Trypanothione reductase (TR) is a suitable target for drug discovery approaches against leishmaniasis, although the identification of potent inhibitors is still challenging. TR structure from different protozoan parasites has been extensively characterized by crystallography, showing that all key residues are conserved. This homodimeric flavoenzyme possesses four cavities binding two nicotinamide adenine dinucleotide phosphate hydrogen (NADPH) and two trypanothione molecules. Each NADPH cavity is separated from the trypanothione active site by a flavin adenine dinucleotide (FAD) cofactor allowing the transfer of two electrons by the participation of two catalytic cysteines (C52 and C57) which, together with H461′, E466′, and E467′ of the γ-Glu site, form the catalytic machinery. The active site features a hydrophobic cleft, named mepacrine binding site (MBS) after the crystal structure with the mepacrine inhibitor was solved.

To validate the predicted binding mode for further rational structure-based drug design and ligand optimization, the structures of TbTR with the most promising compounds 9, 10, and 14 were determined by X-ray crystallography. The effect of N-piperazine substitution on binding affinity was assessed by introducing a methyl or a diClBn group in B to afford quaternary ammonium salts 9 and 10, respectively. Quaternization of the piperazine promotes improvement in IC50 values compared to that of 5 (IC50 = 54.6 μM) by about 3-fold for 9 (IC50 = 20.5 μM), 42-fold for 10 (IC50 = 1.31 μM), and 23-fold for 14 (IC50 = 2.35 μM). However, this improvement does not seem to relate to the interaction between the positively charged ammonium and the protein but as shown in the solved structures, rather to the larger inhibitor structures, more efficiently occupying the binding pocket. Remarkably, 10, endowed with a completely new chemotype and a Ki value of 0.2 μM, stands among the most effective LiTR inhibitors so far developed. The densities observed inside the trypanothione pocket for both TR dimers provided well-defined results for some portions of the compounds, namely, the ethyl-p-fluorophenyl and furan moieties, indicating that these common portions anchor 9, 10, and 14 to the Z-site by van der Waals and electrostatic interactions, as previously observed for fragment. From the interaction network, it is clear that the furan and the ethyl-p-fluorophenyl groups anchor 9, 10, and 14 to the Z-site, consistently with the binding of the initial fragments. It is also evident that the dichlorobenzyl group—when present—protrudes toward the MBS together with the phenylpropyl moiety, making a T-shaped π-stacking interaction with W21. With regard to selectivity, the binding of the optimized fragments 10 and 14 is probably allowed for hGR despite the presence of the bulkier side chains in hGR compared to those in TR.

>[4x]GSHMSKAFDLVVIGAGSGGLEAGWNAATLYGKRVAVVDVQTSHGPPFYAALGGTCVNVGCVPKKLMVTGAQYMDHLRESAGFGWEFDGSSVKANWKKLIAAKNEAVLDINKSYEGMFNDTEGLDFFLGWGSLESKNVVVVRETADPKSAVKERLQADHILLATGSWPQMPAIPGIEHCISSNEAFYLPEPPRRVLTVGGGFISVEFAGIFNAYKPPGGKVTLCYRNNLILRGFDETIREEVTKQLTANGIEIMTNENPAKVSLNTDGSKHVTFESGKTLDVDVVMMAIGRIPRTNDLQLGNVGVKLTPKGGVQVDEFSRTNVPNIYAIGDITDRLMLTPVAINEGAALVDTVFGNKPRKTDHTRVASAVFSIPPIGTCGLIEEVAAKEFEKVAVYMSSFTPLMHNISGSKYKKFVAKIVTNHSDGTVLGVHLLGDGAPEIIQAVGVCLRLNAKISDFYNTIGVHPTSAEELCSMRTPSYYYVKGEKMEKLPDSNL> MSRDRFRSRGGGGGGFHRRGGGGGRGGLHDFRSPPPGMGLNQNRGPMGPGPGGPKPPIPPPPPHQQQPQQPPPQQPPPQQPPPHQQPPPHQPPHQQPPPPPQDSSKP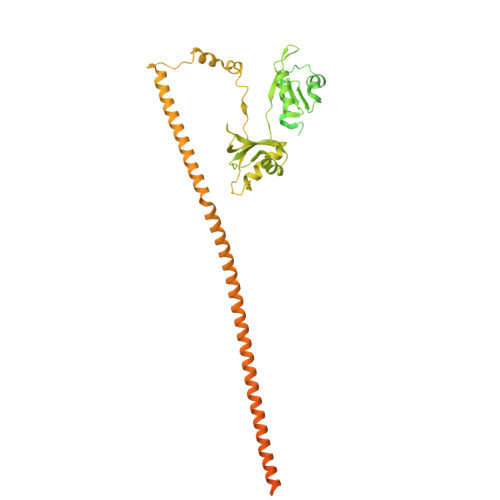VVPQGPGSAPGVSPAPPPAGSAPPANPPTTGAPPGPGPTPTPPPAVTSATPGPPPPSTPSSGVSTTPPQSGGPPPPPAGGAGPGPKQGPGPGPGGPKGGKMPGGPKPGGGPGMGAPGGHPKPPHRGGGEPRGGRQHHPPYHQQHHQGPPPGGPAARTEEKISDSEGFKANLSLLRRPGEKTYTQRCRLFVGNLPADITEDEFKRLFAKYGEPGEVFINKGKGFGFIKLESRALAEIAKAELDDTPMRGRQLRVRFATHAAALSVRNLSPYVSNELLEEAFSQFGPIERAVVIVDDRGRSTGKGIVEFASKPAARKAFERCSEGVFLLTTTPRPVIVEPLEQLDDEDGLPEKLAQKNPMYQKERETPPRFAQHGTFEYEYSQRWKSLDEMEKQQREQVEKNMKDAKDKLESEMEDAYHEHQANLLRQDLMRRQEELRRMEELHSQEMQKRKEMQLRQEEERRRREEEMMIRQREMEEQMRRQREESYSRMGYMDPRERDMRMGGGGTMNMGDPYGSGGQKFPPLGGGGGIGYEANPGVPPATMSGSMMGSDMRTERFGQGGAGPVGGQGPRGMGPGTPAGYGRGREEYEGPNKKPRF> PDITATPAWDALARHHDQIGNTHLRQFFADDPGRGRELTVSVGDLYIDY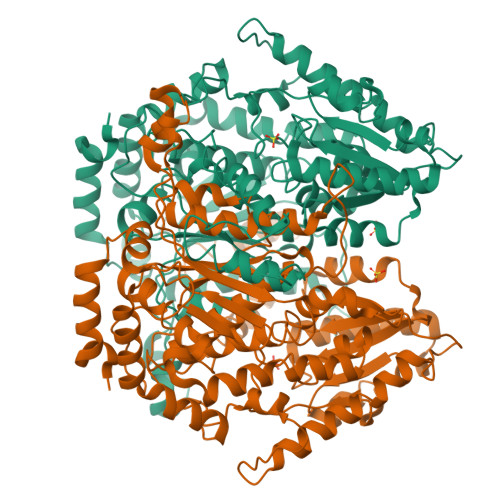SKHRVTRETLALLIDLARTAHLEERRDQMFAGVHINTSEDRAVLHTALRLPRDAELVVDGQDVVTDVHAVLDAMGAFTDRLRSGEWTGATGKRISTVVNIGIGGSDLGPVMVYQALRHYADAGISARFVSNVDPADLIATLADLDPATTLFIVASKTFSTLETLTNATAARRWLTDALGDAAVSRHFVAVSTNKRLVDDFGINTDNMFGFWDWVGGRYSVDSAIGLSLMTVIGRDAFADFLAGFHIIDRHFATAPLESNAPVLLGLIGLWYSNFFGAQSRTVLPYSNDLSRFPAYLQQLTMESNGKSTRADGSPVSADTGEIFWGEPGTNGQHAFYQLLHQGTRLVPADFIGFAQPLDDLPTAEGTGSMHDLLMSNFFAQTQVLAFGKTAEEIAADGTPAHVVAHKVMPGNRPSTSILASRLTPSVLGQLIALYEHQVFTEGVVWGIDSFDQWGVELGKTQAKALLPVITGAGSPPPQSDSSTDGLVRRYRTERGRAGLE>[2x]MREEIGYVPVGEAELYVEDVGPVEGPALFVLHGGPGGNAYVLREGLQDYLEGFRVVYFDQRGSGRSLELPQDPRLFTVDALVEDTLLLAEALGVERFGLLAHGFGAVVALEVLRRFPQAEGAILLAPWVNFPWLAARLAEAAGLAPLPDPEENLKE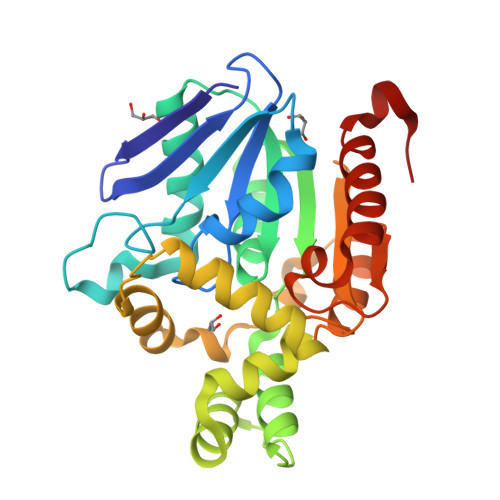ALKREEPKALFDRLMFPTPRGRMAYEWLAEGAGILGSDAPGLAFLRNGLWRLDYTPYLTPERRPLYVLVGERDGTSYPYAEEVASRLRAPIRVLPEAGHYLWIDAPEAFEEAFKEALAALVPALRGPLVD>MVHYKLTYFNGRGAGECARQVFALADQKYEDVRLTQETFVPLKATFPFGQVPVLEVDGQQLAQSQAICRYLAKTFGFAGATPFESALIDSLADAYTDYRAEMKTYYYTALGFMTGDVDKPKTDVLLPARTKFLGFITKFLKK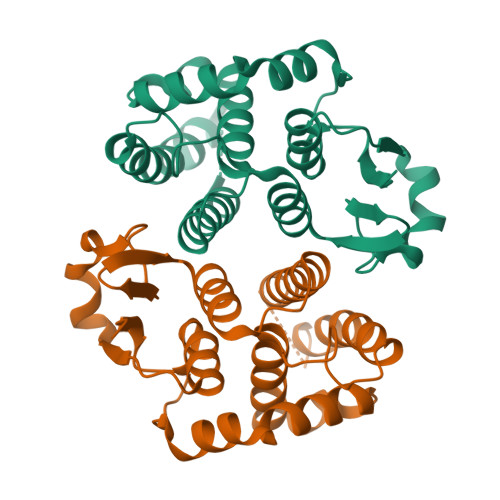NSSGFLVGDKISWVDLLVAEHVADMTNRVPEYIEGFPEVKAHMERIQQTPRIKKWIETRPETPF[8x]Dinucleases of the DEDD superfamily, such as oligoribonuclease, Rexo2 and nanoRNase C, catalyze the essential final step of RNA degradation, the conversion of di- to mononucleotides. The active sites of these enzymes are optimized for substrates that are two nucleotides long, and do not discriminate between RNA and DNA. The active sites invariably consist of (i) a catalytic DEDDh/y-containing core for divalent cation coordination and catalysis, (ii) a leucine residue that wedges between the two bases of the substrates and (iii) a 5′-phosphate cap that coordinates the 5′ phosphate of the dinucleotides. Here, we identified a novel DEDD subfamily, members of which function as dedicated deoxydinucleases (diDNases) that specifically hydrolyze single-stranded DNA dinucleotides in a sequence-independent manner.

To confirm that Actinomycetal Orn proteins function as dinucleases, we measured the in vitro and in vivo activities of Orn from Blastococcus (OrnBla) and Nocardioides (OrnNoc). Actinomycetal Orn proteins readily cleaved both the RNA and DNA dinucleotides in vitro. A comparison of their kinetic parameters with those of previously studied Orn homologs from Gammaproteobacteria V. cholerae and P. aeruginosa, OrnVc and OrnPa, respectively, revealed that OrnVc did not distinguish between RNA and DNA dinucleotides and that OrnPa, OrnBla, and OrnNoc had a slight bias toward diribonucleotides. Given that OrnBla and OrnNoc were able to rescue the small-colony phenotype of the P. aeruginosa Δorn strain to the same extent as OrnPa, our results suggest a conserved cellular role for Orn proteins as housekeeping dinucleases. The crystal structure of OrnBla in complex with pGG further confirmed a conserved mode of substrate coordination across the bacterial Orn family, including homologs from Gram-positive species. Structural superposition of OrnBla-pGG and OrnVc-pGG showed that the sugar-phosphate backbones of the substrates aligned perfectly. Neither structure revealed elements in the active sites that would restrict the space for the 2′OH group of the nucleotide's ribose. The residues of the active sites facing the substrate sugars are hydrophilic and can accommodate both deoxyribose and ribose. The only significant structural difference between OrnBla and OrnVc is the additional C-terminal helix of the former, which is far from the active site and has been previously reported to stabilize the dimeric assembly of Orn from M. smegmatis.

>[8x]SMADSAGHLVWIDCEMTGLDLVEDKLIEVAVLITDSELNVLDPGLDLIISADDAALDGMNEVVRTMHEKSGLTEEVRASTLTVAEAEQQVLAYIKRWVPERRTAPLCGNSIGTDRGFLARDMPELDDHLHYRMIDVSSVKELARRWFPRVYFGQPAKGLAHRALADIIESVRELAYYRRTVFVDSPGPSSSQAKKAAAEVVGGFAALLDGDEKAPAPGA>[4x]AESLPDLKIEKLDEGVYVHTSFEEVNGWGVVPKHGLVVLVNAEAYLIDTPFTAKDTEKLVTWFVERGYKIKGSISSHFHSESTGG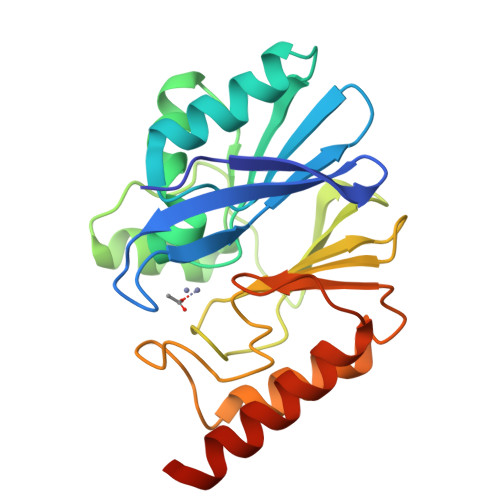IEWLNSRSIPTYASELTNELLKKDGKVQATNSFSGVNYWLVKNKIEVFYPGPGHTPDNVVVWLPERKILFGGCFIKPYGLGNLGDANIEAWPKSAKLLKSKYGKAKLVVPSHSEVGDASLLKLTLEQAVKGLNESKKPSKPSN> SPQPLEQIKLSESQLSGRVGMIEMDLASGRTLTAWRADERFPMVSTFKVVLCGAVLARVDAGDEQLERKIHYRQQDLVDYSPVSEKHLADGMTVGELCA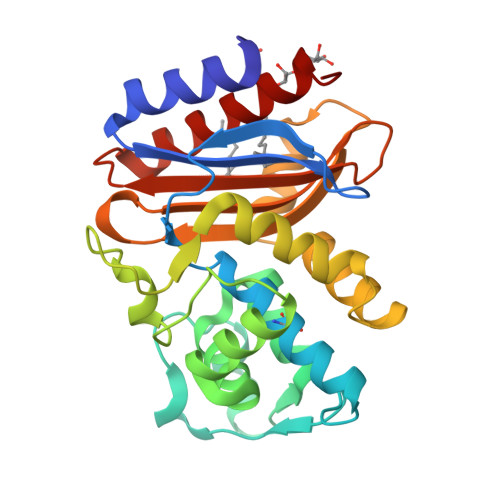AAITMSDNSAANLLLATVGGPAGLTAFLRQIGDNVTRLDRWETELNEALPGDARDTTTPASMAATLRKLLTSQRLSARSQRQLLQWMVDDRVAGPLIRSVLPAGWFIADKTGAGERGARGIVALLGPNNKAERIVVIYLRDTPASMAERNQQIAGIGAALIEHWQR>GSHMSGSKEEVPDNPPNEIYATAQQKLQDGNWRQAITQLEALDNRYPFGPYSQQVQLDLIYAYYKNADLPLAQAA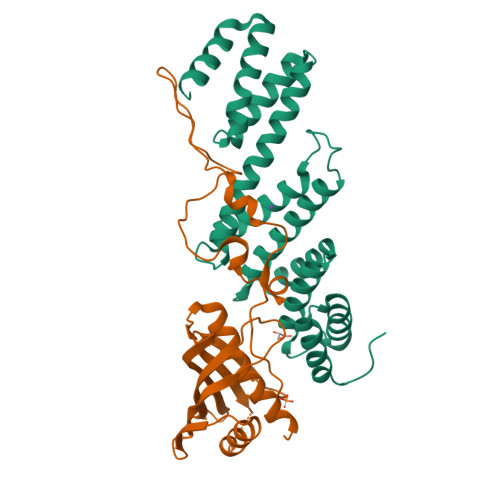IDRFIRLNPTHPNIDYVMYMRGLTNMALDDSALQGFFGVDRSDRDPQHARAAFSDFSKLVRGYPNSQYTTDATKRLVFLKDRLAKYEYSVAEYYTERGAWVAVVNRVEGMLRDYPDTQATRDALPLMENAYRQMQMNAQAEKVAKIIAANSSNT[2x];>[2x]GSHMSSDSRYKRQVSGDEAYLEAAPLAELHAPAGMILPVTSGDYAIPVTNGSGAVGKALDIRPPAQPLALVSGARTQFTGDTASLLVENGRGNTLWPQVVSVLQAKNYTITQRDDAGQTLTTDWVQWNRLDEDEQYRGRYQISVKPQGYQQAVTVKLLNLEQAGKPVADAASMQRYSTEMMNVISAGLDKSATDAANAAQNRASTTMDVQSAADDTGLPMLVVRGPFNVVWQRLPAALEKVGMKVTDSTRSQGNMAVTYKPLSDSDWQELGASDPGLASGDYKLQVGDLDNRSSLQFIDPKGHTLTQSQNDALVAVFQAAFSK> MSKDYQSLANLSPFELKDELIKIASGDGNRLMLNAGRGNPNFLATTPRRAFFRLGLFAAAESELSYSYMNTVGVGGLAKIEGIEGRFERYIAENRDQEGVRFLGKSLSYVRDQLGLDPAAFLHEMVDGILGCNYPVPPRMLNISEKIVRQYIIREMGADAIPSESVNLFAVEGGTAAMAYIFESMKVNGLLKAGDKVAIGMPVFTPYIEIPELAQYALEEVAINADPALNWQYPDSELDKLKD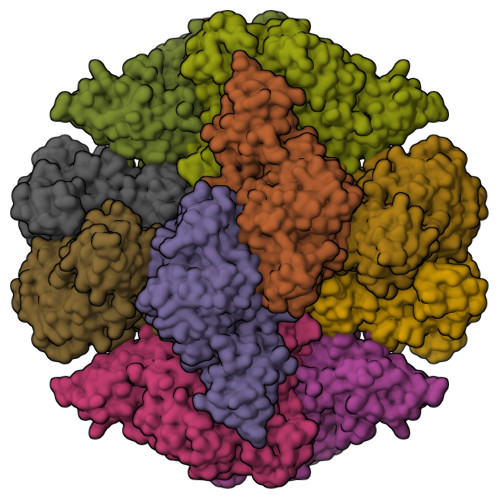PAIKIFFCVNPSNPPSVKMDERSLERVRKIVAEHRPDLMILTDDVYGTFADGFQSLFAICPANTLLVYSFSKYFGATGWRLGVVAAHKENIFDLALGRLPESEKTALDDRYRSLLPDVRSLKFLDRLVADSRAVALNHTAGLSTPQQVQMTLFSLFALMDESDQYKHTLKQLIRRREATLYRELGTPPQRDENAVDYYTLIDLQDVTSKLYGEAFSKWAVKQSSTGDMLFRIADETGIVLLPGRGFGSDRPSGRASLANLNEYEYAAIGRALRQMADELYAQYTQQGNKR>[2x]MTTSESPDAYTESFGAHTIVKPAGPPRVGQPSWNPQRASSMPVNRYRPFAEEVEPIRLRNRTWPDRVIDRAPLWCAVDLRDGNQALIDPMSPARKRRMFDLLVRMGYKEIEVGFPSASQTDFDFVREIIEQGAIPDDVTIQVLTQCRPELIERTFQACSGAPRAIVHF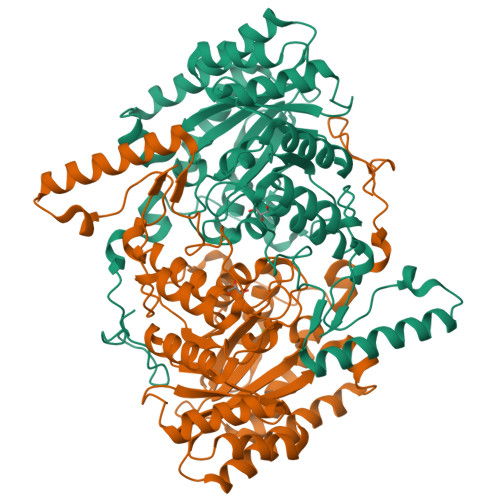YNSTSILQRRVVFRANRAEVQAIATDGARKCVEQAAKYPGTQWRFEYSPESYTGTELEYAKQVCDAVGEVIAPTPERPIIFNLPATVEMTTPNVYADSIEWMSRNLANRESVILSLHPHNDRGTAVAAAELGFAAGADRIEGCLFGNGERTGNVCLVTLGLNLFSRGVDPQIDFSNIDEIRRTVEYCNQLPVHERHPYGGDLVYTAFSGSHQDAINKGLDAMKLDADAADCDVDDMLWQVPYLPIDPRDVGRTYEAV> MAHHHHHHSSGLEVLMDAPMEDAPAPVAQVKVIFTTTEPDLELPESKRQLLVPADIRRYGLSRILNSESMLDTGSIPFDFLINGSFLRSSLEDYLTSNGLSLETTLTLQYVRSLIPPVYEASFEHDDWVSAVDVLSATSPAGRWSSAANSSAAVQPGQERVLSASYDGLLRIWNASGSVIATSPSGSHGGHTASIKAAKFLTSDRLASAGMDRTVRVWKYTESDHFTGELKPTLELYGHTGSVDWLDVDGHSKHILTASADGAIGFWSASKASAPEPDASLLPGAHVSKRRKATSSVSTAQRGPLGLWSIHTAPATAAIFD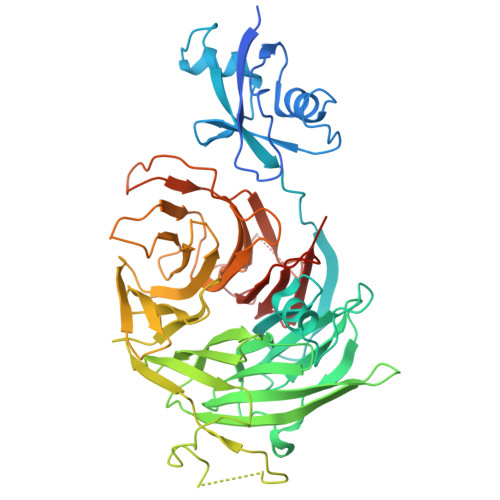PRDRTVAYSASQDHTVRTLDLTTGQVVSTLTLTHPLLSLSALTRAGTTSPLLAAGTSARHITMVDPRASSATTSVMTLRGHANKVVSLSPSPENEYSLVSGSHDGTCRVWDLRSVRPATKEEGSLGGVSEPVYVIERESWASKGKKKRPVAGDGCKVFSVVWDKLGIFSGGEDKKVQVNRGRNIVTEQK>SEILRYLM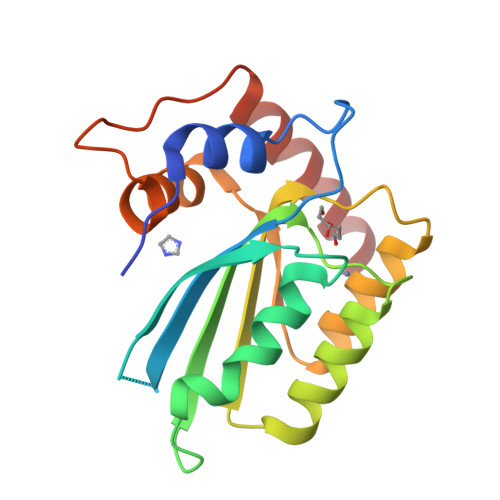DPDTFTSNFNNDPLVLRRRQTYLCYEVERLDNGTSVKMDQHMGFLCNESGRHAELRFLDLVPSLQLDPAQIYRVTWFISWSPCFSWGCAGEVRAFLQENTHVRLRIKAARIYDYDPLYKEALQMLRDAGAQVSIMTYDEFEYCWDTFVYRQGCPFQPWDGLEEHSQALSGRLRAILQ[2x]>MKNITIYTKNYCPYCKKAVSLLSSKGVDFKEVDVTHDSKAFEDVMAKTGWDTVPQVFVDEEFLGGCDDI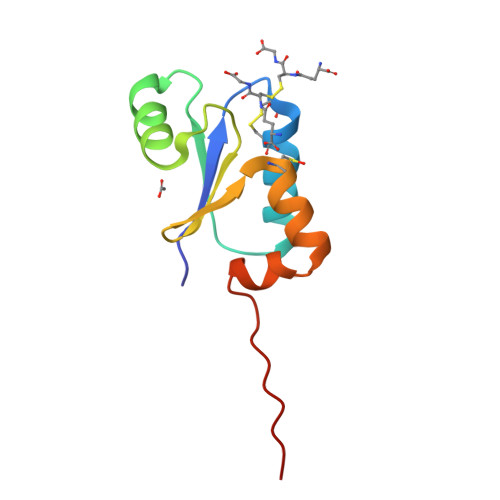HALDRQGILDKKLGLKLEHHHHHH[2x]>GHHHHHHVPAFLTKLWTLVSDPDTDALICWSPSGNSFHVFDQGQFAKEVLPKYFKHNNMASFVRQLNMYGFRKVVHIEQGGLVKPERDDTEFQHPCFLRGQEQLLENIKRKVT[6x]

Heat shock factor 1 (HSF1) and 2 (HSF2) play distinct but overlapping regulatory roles in maintaining cellular proteostasis or mediating cell differentiation and development. Upon activation, both HSFs trimerize and bind to heat shock elements (HSEs) present in the promoter region of target genes. HSFs recognize and bind HSEs through the DBD, which is the most conserved and only structurally characterized domain. Here, we present co-crystal structures of human HSF1 and HSF2 trimers bound to DNA, which reveal a triangular arrangement of the three DNA-binding domains (DBDs) with protein-protein interactions largely mediated by the wing domain.

Crystallization of the HSF1 trimer in complex with the same three-site HSE was unsuccessful until longer sticky-ended DNA duplexes were attempted. Two structures containing 23- and 24-bp oligonucleotides were determined and refined at 2.4 and 2.36 Å. Different from the HSF2 structure, two HSF1 trimers bound to two intact HSEs reside in the asymmetric unit in both structures, where the DNA duplexes were stacked in a head-to-head manner. As a consequence, the two HSF1 trimers are differently oriented with a large rotation angle between them, but little conformational discrepancies exist among all the HSF1-HSE copies present in both structures. Like HSF2, Arg117 (corresponding to Arg109 in HSF2) in the middle DBD (DBD II) also inserts into the major groove and forms a direct hydrogen bond with the nucleobase 5′ to TTC. For example, in the structure comprising 23-bp DNA, the C terminus of DBD II in the first trimer is rigidified by a close contact between Lys118 and the phosphate backbone of DNA but not in the other two DBDs. In contrast, such an electrostatic contact is observed in multiple DBDs in the other structure containing 24-bp DNA. Apart from a purine with an imino nitrogen participating in the contact, the amino nitrogen outside the pyrimidine ring in cytosine may also engage in an indirect hydrogen bond, which, however, is only present in the structure of HSF1 bound to 24-bp DNA that shows more pronounced DNA bending than the other HSF1 structure. Based on these observations, we reason that cytosine is a less favorable nucleobase than a purine at this position because its amino nitrogen is barely positioned at an indirect hydrogen bonding distance with the Asn residue only in a context with sufficient DNA backbone distortion. By contrast, in both HSF1 trimer-binding structures, dramatic bending occurs at both the 5′-proximal HSE triplet and the downstream dinucleotide, although relatively smaller bending occurs at the 3′-proximal nGAAn repeat bound by DBD III.(2~{R})-~{N}-[3-[2-[[(2~{S})-2-formamido-3-methyl-butanoyl]amino]ethylamino]-3-oxidanylidene-propyl]-3,3-dimethyl-2-oxidanyl-4-[oxidanyl-bis(oxidanylidene)-$l^{6}-phosphanyl]oxy-butanamide 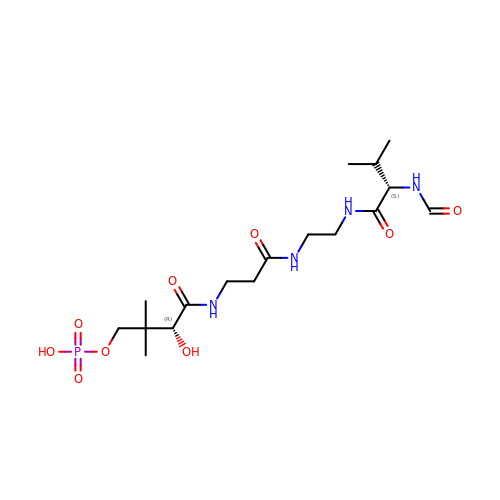| C17 H32 N4 O9 P | SZJRFDKIBVCSLN-KBPBESRZSA-N(2S,3R,4S,5R,6R)-6-(hydroxymethyl)-4-undec-10-enoxy-oxane-2,3,5-triol 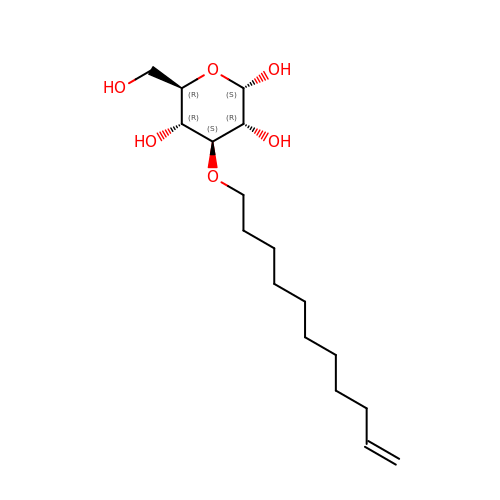| C17 H32 O6 | YZRNUMHABGDGTN-MTSZKFMLSA-N> MVLLHKSTHIFPTDFASVSRAFFNRYPNPYSPHVLSIDTISRNVDQEGNLRTTRLLKKSGKLPTWVKPFLRGITETW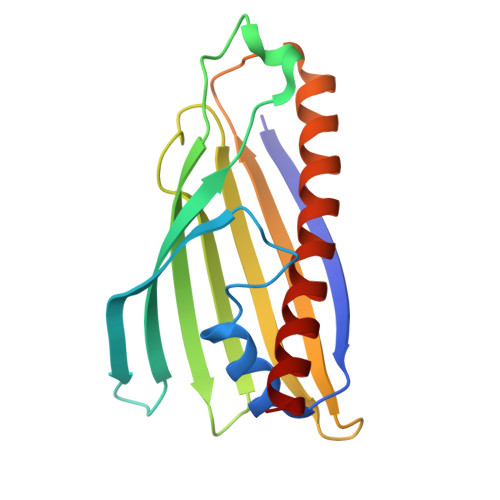IIEVSVVNPANSTMKTYTRNLDHTGIMKVEEYTTYQFDSATSSTIADSRVKFSSGFNMGIKSKVEDWSRTKFDENVKKSRMGMAFVIQKLEEA>[2x]GSERPKLDEGFYEIEAIRRKRVRKGKVQYLIKWRGWPETANTWEPLENLQSI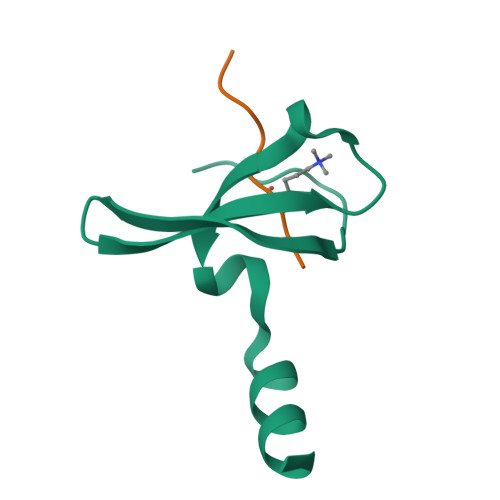ADVIDAFEGSLKPG;>[2x]ARKSAPTT> GSHMASPNGQTKPLP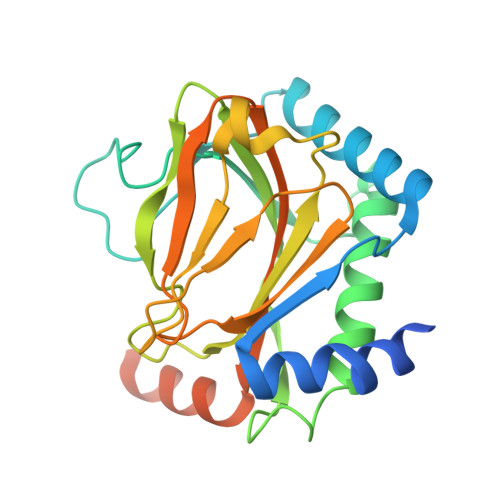ALKLALEYIVPAMNKHGICVVDDFLGKETGQQIGDEVRALHDTGKFTDGQLVSQKSDSSKDIRGDKITWIEGKEPGCETIGLLMSSMDDLICHCNGKLGSYKINGRTKAMVACYPGNGTGYVRHVDNCNGDGRCVTCIYYLNKDWDAKVSGGILRIFPEGKAQFADIEPKFDRLLFFWSDRRNPHEVQPAYATRYAITVWYFDADETAAAKVKYLTGEKGVRVELNKPSDSVGKDVF>[4x]SFDCGKPQVEPKKCPGRVVGGCVAHPHSWPWQVSLRTRFGMHFCGGTLI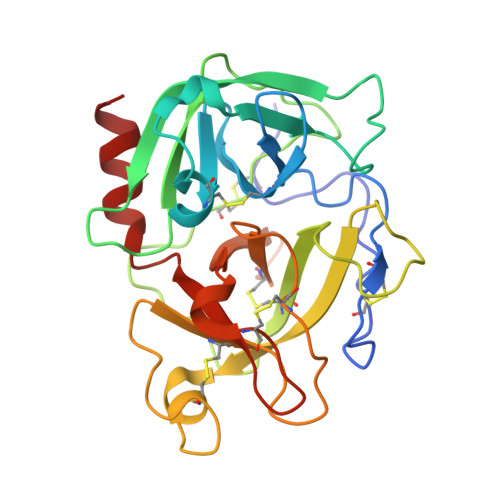SPEWVLTAAHCLEKSPRPSSYKVILGAHQEVNLEPHVQEIEVSRLFLEPTRKDIALLKLSSPAVITDKVIPACLPSPNYVVADRTECFITGWGETQGTFGAGLLKEAQLPVIENKVCNRYEFLNGRVQSTELCAGHLAGGTDSCQGDAGGPLVCFEKDKYILQGVTSWGLGCARPNKPGVYVRVSRFVTWIEGVMRNN> SMSGAGEGQGPKKQTRLGLEAKKEENLADWYSQVITKSEM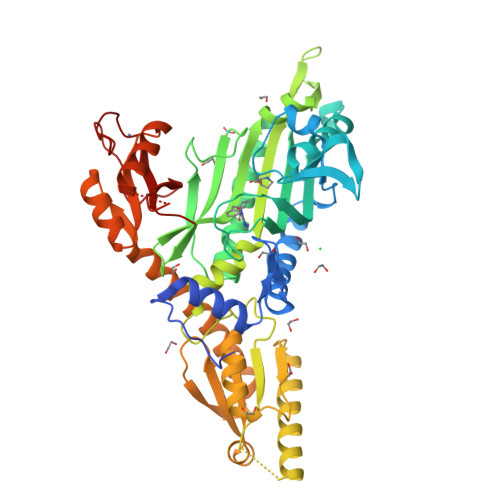IEYHDISGCYILRPWAYAIWEAIKDFFDAEIKKLGVENCYFPMFVSQSALEKEKTHVADFAPEVAWVTRSGKTELAEPIAIRPTSETVMYPAYAKWVQSHRDLPIKLNQWCNVVRWEFKHPQPFLRTREFLWQEGHSAFATMEEAAEEVLQILDLYAQVYEELLAIPVVKGRKTEKEKFAGGDYTTTIEAFISASGRAIQGGTSHHLGQNFSKMFEIVFEDPKIPGEKQFAYQNSWGLTTRTIGVMTMVHGDNMGLVLPPRVACVQVVIIPCGITNALSEEDKEALIAKCNDYRRRLLSVNIRVRADLRDNYSPGWKFNHWELKGVPIRLEVGPRDMKSCQFVAVRRDTGEKLTVAENEAETKLQAILEDIQVTLFTRASEDLKTHMVVANTMEDFQKILDSGKIVQIPFCGEIDCEDWIKKTTARDQDLEPGAPSMGAKSLCIPFKPLCELQPGAKCVCGKNPAKYYTLFGRSY> GS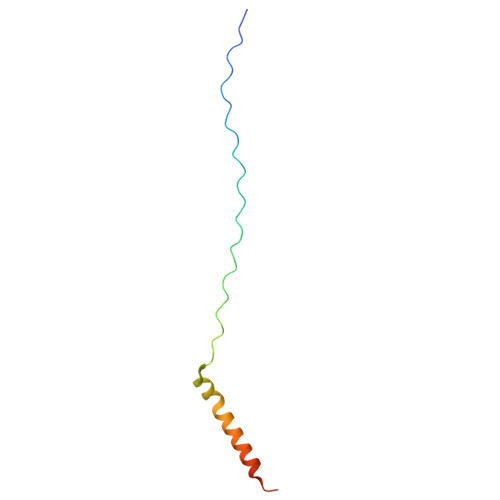GPPGPPGPPGPPGARGQAGVMGFPGPPGPPGPPGKEASEQRIRELCGGMISEQIAQLAAHLRKPLAPGSI>KQVAGYYQYQAGDVQITALLDGTNFMSPNLFKDIPQQQVHEILKKYY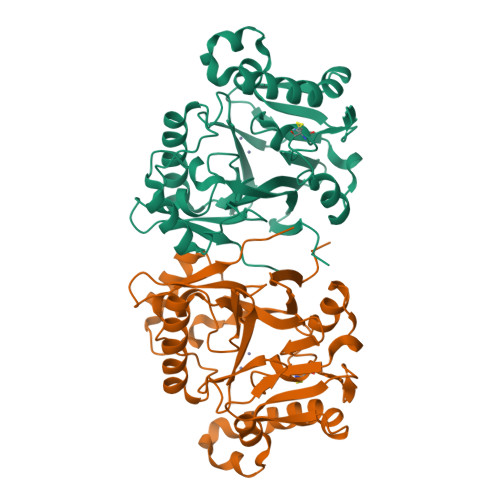ADQEKGVQTSINAFLVNIGKSLILIDSGAASCFGSHLGSVLSNLKASGYQPEQVDTILLTHLHPDHVCGISKDGVANFPNATVYVSNDEASFWLDPKQAAKLPKEKQANYLGTVEKIKQAIAPYQAKQRFKTYKLGDDIQGFKVINTAGHTPGHFSYELKTKGESIVFIGDIVHSHTVQFDRPETAIEYDIDPKKAVETRLKQFANFAKNGQTIAAPHLPFPGIGHTYSADGKSYQWIPIHFKD[2x]CAP (catabolite activator protein) is a DNA-binding protein and transcription activator that recruits RNA polymerase to more than 100 genes in Escherichia coli. The CAP dimer consists of two identical 209-residue subunits, each with an N-terminal binding domain for allosteric effector cAMP, and a C-terminal winged helix–turn–helix DNA-binding motif. CAP has three defined ‘activating regions’, patches of surface-exposed residues that interact with RNA polymerase (RNAP) in specific CAP-dependent promoter classes.

The crystal structure of cyclic AMP–catabolite activator protein (CAP) from Escherichia coli containing cobalt(II) chloride and ammonium sulfate is reported at 1.97 Å resolution. We describe here the structure of cAMP–CAP in a novel fourth crystal form (space group P21212 with one dimer in the asymmetric unit) in which cobalt(II) binds to key residues of CAP AR2. The crystal asymmetric unit contains one CAP dimer (residues 7–207 of chain A and 7–206 of chain B were modeled out of 210 total residues per subunit), with cAMP ligands bound as expected within the N-terminal domain, two cobalt(II) cations, 13 sulfate anions and 420 solvent atoms. The conformation of the CAP dimer in this new crystal form is essentially identical to the conformation observed in earlier structure reports for cAMP–CAP, with two cAMP-binding N-terminal domains related by local twofold rotational (C2) symmetry, and flexibly tethered DNA-binding C-terminal domains that adopt two distinct positions relative to the N-terminal domains. Each of the two CAP subunits in the asymmetric unit binds one cobalt(II) ion, in each case coordinated by N-terminal domain residues His19, His21 and Glu96 plus an additional acidic residue contributed via a crystal contact. In each case, a neighboring CAP dimer related by crystal symmetry contributes two additional ligands from residue Glu37 (O∊1 and O∊2). Octahedral coordination is completed at each site by a solvent water O atom. The three N-terminal domain Co2+-binding residues (His19, His21 and Glu96) constitute a major subset of the four residues previously identified to form CAP activating region 2 (AR2), which participates in transcription activation specifically at class II CAP-dependent promoters. Sulfate anions mediate additional crystal lattice contacts and occupy sites corresponding to DNA backbone phosphate positions in CAP–DNA complex structures. The DNA in the CAP dimer–DNA complexes is strongly bent and electrostatic interactions are thought to play an important role in DNA bending; our structure suggests that the CAP C-terminal domains have an intrinsic capability to bind to DNA half-sites prior to adoption by CAP of its fully bent DNA binding conformation.

>[2x]VLGKPQTDPTLEWFLSHCHIHKYPSKSTLIHQGEKAETLYYIVKGSVAVLIKDEEGKEMILSYLNQGDFIGELGLFEEGQERSAWVRAKTACEVAEISYKKFRQLIQVNPDILMRLSAQMARRLQVTSEKVGNLAFLDVTGRIAQTLLNLAKQPDAMTHPDGMQIKITRQEIGQIVGCSRETVGRILKMLEDQNLISAHGKTIVVYGTR>[4x]MTTPSMEDYIEQIYMLIEEKGYARVSDIAEALAVHPSSVTKMVQK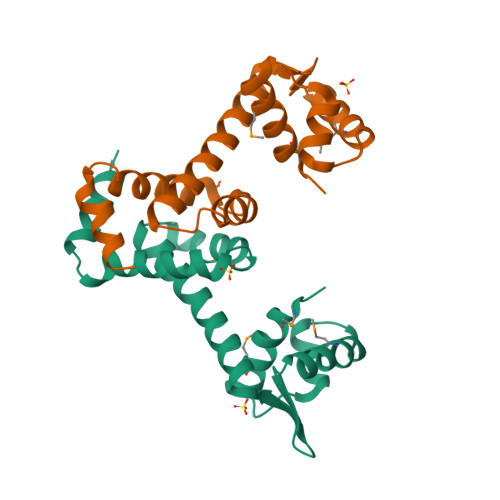LDKDEYLIYEKYRGLVLTSKGKKIGKRLVYRHELLEQFLRIIGVDEEKIYNDVEGIEHHLSWNSIDRIGDLVQYFEEDDARKKDLKSIQKKTEHHNQ Milano is a contractile tail bacteriophage that infects the pathogenic plant bacterium Agrobacterium tumefaciens, an important tool that is widely used in genetic manipulations of plants. The contractile tail of Agrobacterium tumefaciens bacteriophage Milano is flexible and bent to varying degrees, which sets it apart from other contractile tail-like systems. A contractile sheath and rigid tube assembly is a widespread apparatus used by bacteriophages, tailocins, and the bacterial type VI secretion system to penetrate cell membranes. In this mechanism, contraction of an external sheath powers the motion of an inner tube through the membrane.

We have determined the structure of the distal part of the tail comprising the baseplate with associated receptor-binding proteins (RBPs) and two baseplate-proximal layers of the sheath-tube complex to ~3.2 Å resolution. Tail-sheath, tube, baseplate centerpiece (BCP), baseplate wedge (BW), and receptor-binding complex (tail-spike + short tail-fibers + garland) are arranged in C6 symmetry, while baseplate hub (BH) and baseplate central spike (BCS) have a C3 symmetry. The structure of the central spike complex of Milano, which consists of BH and BCS proteins, is similar to that of the central spike complex of R-type pyocin (PA0628–PA0616)17 and phage T4 (gp27–gp5)48. A similar Fe ion is likely present in the Milano BCS because the cryo-EM map of the Milano baseplate shows a spherical peak of 6.5 standard deviations above the mean between the side chains of His166 and His168 matching the expected location of a Fe ion. Similar to the T4 and R-type pyocin baseplate proteins, BW2 (T4 gp6, pyocin PA0618) and BW3 (T4 gp7, pyocin PA0619) form a (BW2)2–BW3 heterotrimer. The similarity of the Milano BCP organization to that of the pyocin (PA0626) suggests its central role in the function of the baseplate. In addition to the BW4 C-terminal domain mentioned above (residues 346–396), the Milano BCP protein contains an N-terminal Tube domain (residues 1–127) and a middle Helical domain (residues 141–345). Similar to the tail-sheath assembly, the Milano baseplate also features an extensive disulfide bond network. Considering that the BCP must leave the baseplate to allow the tube to move and sheath to contract and that the wedges of the Milano baseplate might be required to splay out to initiate sheath contraction, the baseplate disulfide bond network must be almost entirely disintegrated prior to sheath contraction. The Milano RBP complex contains no such fiber but includes at least four different types of proteins—TSP (gp124), STF (gp31), and garland (gp125 and gp127) that are connected to each other.

> MTTSKTYDERNRDIQDGFERHVFKGIEHTDTGALVSVKGSGTQEEDVPVINSGYGFTPAADTELEVFLHGDGSDASNKFATMTIPRNKQRKWPEGAGGVQHPFNADKFVQFDDDSIWLKDGKFTLGNNQELTITVSNGLVTLSSNNEVDFRCPKLMHNGVNIGDSHVHPQKPDSGGDSEEDTDPPKRD;> MIKPMRIFIGGEELVTYTSAQLQRTKKQMTGSLTVEIFLDYVPTKPTIVNAVRGKEILVYIMGELAFTGIIDKRRGKSVKKQNRDASGRFAFSGGPGSLSEDAGGDVSVNFSKGNGYSVTLTARGRTKYLIDSSQTHPTGFFKNTSDKKVIETLVKEHNVVLQWDAEEIDEPKVTLRDGNRIYNEIFERCNQNCHFAYETRDGKLLITDGTNGTVGEDIILGYNILDFSAEQSEDQANSQITVKGHRTQKGVWGNDAIVQPVQTVADSWVGANIPLTIQHYGDATNEGLQRRAKFEADRRAAESKSVSVTVFHVAQQTGTPWDIGTVHYVEIPPEGIFDVLECVSLTYTVDAKSTLETKLELAPPPSQGISGGAASGVSGLLSSANNLLSDLTTKGIARRVQAGVQIIGGQYPSSWTSAALSAIANPINAITSVVNSLLAKEDEKPPKQPPMRLPPE;>[4x]MACNKQNGVKNILITFTDCDTQEVIGPISHEQPDDTLPTYKNCAWTNTALTNGYVQRSASNATMTLPVVRDLRVPLAFYQGCAQVDVQVEKFDGTVMTLTEGAVVEPEESDGRSVTMNIVASEIDELLPPGSLAAA;>[4x]MSCTIQRPDPQDLRNDIATRFSTNVLGGAPIIPESNEFYVVSLEYAMQEEFYAFGEQMWRERDPRFACCENLVKMAAERGVYPKPAQFAQGYVRMTGTPGSALNQGLRFQFGNQTYEPASVVPDQLPATGILVLRVSAVNPGPSGNARVTDGTLVTPVPGISSAVTAYGGNFCGGSDEEECEQFRTRYLQRLQYQPRFTVEWLKSKAAEWPCVTDVFDLGPNCCAVNALGEVVCPNNFEFYVLFRDTFDCGLAPQCVVDEITDWLFGSPQGLGLGEAEFGICGKVRTAAPVKLDIILDGLSCATPAQSRVVEERVTDFVNRLPPSTNLTIDQLRFIGLQVLGPSFNFNVAIRSPNDAVQPGLRFTSCGDAEIDCDYKACLNSVVVINNNVTTSGCL;>[2x]MTCTVDVADRRKRFWTTQIAACGTSSDDCGDCARPGLQLMCNGQGQVTVSTDNYAVGLALNILLTDASKADTGCGWTPGNRGGFWGDSFRSDNLRSGSKIRQVPTRTSMRETVSLIRAYALDDLKKLVTYGVAKSVDVDLTYRGSNKIDMTVIIQGVDGNESRVGLTGERISNAWVWS;>[4x]MAQDALSDGFVRLCIDPSLNFFGEGCKILVEGQMTDDGSATPDAVTCVTSELDIIERFGQGSVLTESLRKVFCTCKSGVSVYALPREDAAAGVKAVYTLTIAGPATTDGRVQLYMGEAEYAVDIGVDAGDTATDIAAAIVAAISPDFPYAATAAAGVITLTARNAGTIGNHLSVIYTNLGSCTSVTPEGVTVTFAQTTAGSVNPTPNDYATVVNECCFAVYVLSSDDTDWQENLRDWIRSAWDCSKPQCFGHGYVFNKGTLGQVLADGDNSAELSRLALPTTYPVLPYLTNAAYGALSACSTCNNPELNIQGQTFGLLSCINMPESCTPGWTFGEVTQLQANGFVVSGPSTTSGQGNYTSPYIYNDVTNYLRDEKNRPNATFRDASSRRLAAATGVALAEFLQQFNGLAVFTKNTNIRTGIIGTNPRLMLGKIRKWAQDNVGTLFSEFDNINEDIQLLTDFEVQPKCVGQPGIFHLNMRYRPPVRGARINVNMAPALFDNCDR;>[2x]MNVLIPGIDGMVSAGTLEYTGCCPPSFADVDECTLATAFVGLLPSGPLWDRPKYEAITTITEAGNCAACWTTDHCPTLVDYAVNVGARLASVIERTIWPAVRESDPFTAVTSTADWLNRFDWVNCFETSCRSKELGEKTPIEYMTDCGPVYVKITYPPSLQQAFESALIKSLERLSMGIIKNLAAINFVIEPLKVRVVPVDTTDACENETLCVVLEKTSDFFDGVNANTCGIPTPVAAYIDRDVMQLPSDLDKYIWPGHMAAECIVRSLLSHVSRFCLIRTEQAPD;>[6x]MAKLRPLQVGGVPGCANIPGGEDCQCWPEWTADNGYFFGDVVQQGGVLYYATRDVPPGTPFLAADWAPYRPAATAIPPHNENSTYFQYQPVAYNDKLYTARTDLPPGPFDPANWQEISVEGLVEVVDSATIDFTGTGAAGDPVSADVKLDPDPDNLLSATANGLILTADNIPFPDPSQILISEEVTLRVDYVTGDDATADGTLAKPFATVSAAIGVATTGDRVEIYPGTYIGNFAPKSDVTVVGLEGVVIDGDVTIAAGVSGALVDGLFVDGSVLVNGANGSVTFRNSRVTENVLATGNNTGVYRFENCDIETAAIVNGTGNAEFIFSGGVSENDFFLNSPGTMIVENRSRVKAVLHEAGNMIVQNIGVIESLASTPDNGFLAVMSSSLFDPLTSTYGTISKTGLCPFVFQDFGRDNTDTTALNGPKFIVSNGRDVHGNYDPAFYALPNGQTLNSHFAGIDAALETLQEYSPLDRLVPVDLGFSFTGGWTDGETIGAHVVSRSTIVPENMAGSVFSTDSSTLDGVLNIVVGPSVVGTVTIVDGIATFASSSFNLDPGQTVRVVTTSDGTFDYAALTLVGHREVVYVN;>MAGIFFSGGLACNLTVNAACGIATTGDDCPALYYPPKCNVQVDPLQMNAVISEIANAINAFGNTYDCSRLDNLKQVLNRARNICDLPPFGDAPDMDDRIAGCFDGQSSTVTVQQLVNLVLGQVGTLCQLPQIGAIQDDDWLAGCIDGAARIVPFAAVRSALGGGGGVIGGVIPQNQLFDSWRAGGFWDVSQSTAGRTAFVFRSRKEGIGITVSELFIATGGGAYQSISEWEPSTFAYVPTGETTAIDGGRIQAVAIAFKKGNQWYAKAGDIILPLGGDDGVIRVRTPGYQRLQIWDGVQV[12x];>[2x]MAGPCYNPDAEYLPASFKGFSFDADSSDSDHGRNGAEAEFVFGERTGYADLGIKIKSYQLRARFQTNDHIAQTNAFIAVLESPGPGLLVHPTRGTVFAACRSARVTDSKVDAAGVTYVELDFVEANSVLSGFGLVGNLVALALAPIITATEGSFKRHFSPDNIRYYNTEAVVSTMAQAVTQVQNAYLAISGNDTSQDKWTTVRDFRNVLIDEFTFYSPANAWNVLRNGFAILDAAATGSDKFNVLRNLINWSSTHSDLDGESGDAENAIFTAVRVLSAAYLAKAYTETAATTVNEGLTQYDLIAAVLEQEAQIAKDDCHDNEFFLQIRAFAVDVARVMVNRAYNSPSLIVYAFPGTVHGLVAAWEIFGDAKRSRDLEARNNGSPWAVGPKIISERVRA>MNQCPTDWEAEGDHCYRFFNTLTTW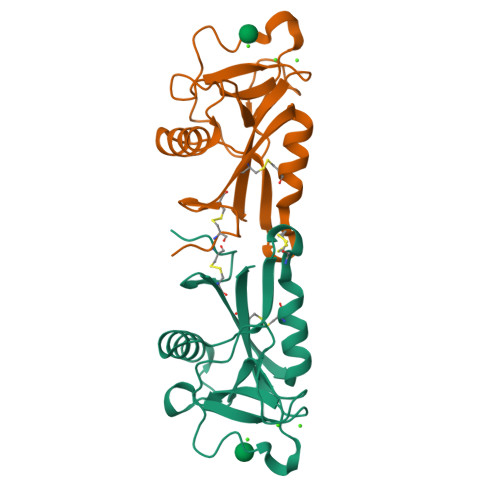ENAHHECVSYSCSTLNVRSDLVSVHSAAEQAYVFNYWRGIDSQAGQLWIGLYDKYNEGDFIWTDGSKVGYTKWAGGEPNNHNNAEDYGQFRHTEGGAWNDNSAAAQAKYMCKLTFE[4x]> GSPGISGGGGGSHIEGYECQPIFLNVLEAIEPGVVCAGHDNNQPDSFAALLSSLNELGERQLVHVVKWAKALPGFRNLHVDDQMAVIQYSWMGLMVFAMGWRSFTNVNSRMLYFAPDLVFNEYRMHKSRMYSQCVRMRHLSQEFGWLQITPQEFLCMKALLLFSIIPVDGLKNQKFF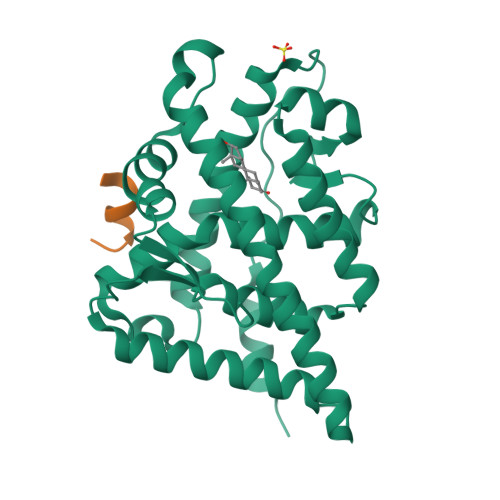DELRMNYIKELDRIIACKRKNPTSCSRRFYQLTKLLDSVQPIARELHQFTFDLLIKSHMVSVDFPEMMAEIISVQVPKILSGKVKPIYFHTQ;> SRFADFFRNEGLGSRSGSGK>DVSGTVCLSALPPEATDTLNLIASDGPFPYSQDGVVFQNRESVLPTQSYGYYHEYTTITPGARTRGTRRIITGEATQEDYYTGDHYATFSL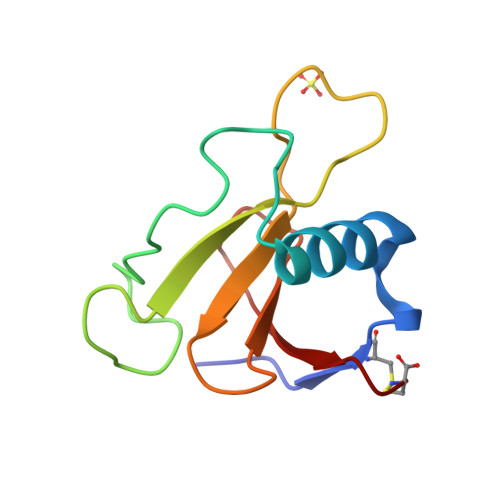IDQTC[2x]> GSHMLPKELQLYFDKILSMIKSDMKDIAIECLEKESGLQQLVPYFIQHISELILKSFKEAEVLKTCIALYFSLIKNKHVFIDPYLHQILPSLLTCVIGKSIVDDDVRKMSADIVKYIYDTYSRSYKTLAPRVLKTLK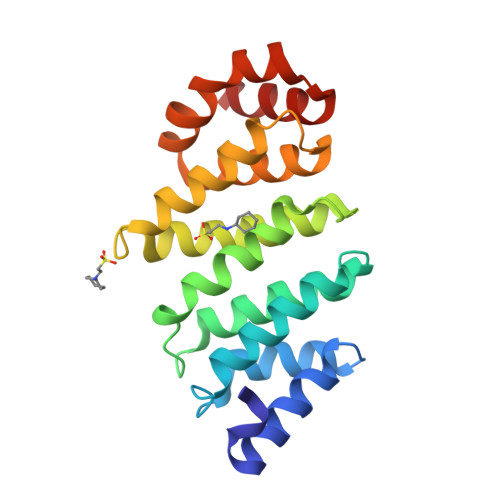GVWMDPNRSEDSQYGALYCLSILSKNVVNTVIREHAEEYKRTIGKKKVTNLLDNVLNVH>MDRRSFITKAAVGGAAASALAAPALAQSAPKVTWRLASSFPKSLDTIFGGAEVLSKMLSEATDGNFQIQVFSAGELVPGLQAADAVTEGTVECCHTVGYYYWGKDPTFALAAAVPFSLSARGINAWHYHGGGIDLYNEFLSQHNIVAFPGGNTGVQMGGWFRREINTVADMQGLKMRVGGFAGKVMERLGVVPQQIAGGDIYPALEKGTIDATEWVGPYDDEKLGFFKVAPYYYYPGWWEGGPTVHFMFNKSAYEGLTPTYQSLLRTACHAADANMLQLYDWKNPTAIKSLVAQGTQLRPFSPEILQACFEAANEVYAEMEASNPAFKKIWDSIKAFRSEHYTWAQIAEYNYDTFMMVQQNAGKL[4x]

In Rhodobacter sphaeroides, TakP (previously named SmoM) is an ESR from a TRAP transporter and binds α-keto acids in vitro. In this paper, we present the high resolution structures of TakP in its unliganded form and complexed with sodium-pyruvate. This study reveals a key role for an ion in the attachment mode of the substrate, as well as an unexpected dimerization largely mediated by a helix swapping. Thus, and despite very low sequence similarity, the TakP fold is characteristic of a type II ESR.

The structure of the selenomethionine-labeled protein in its native form was first solved by the MAD method and then refined to 2.0 Å resolution with an R-factor of 17.9% (Rfree = 20.5%). For the pyruvate complex all the residues fall in the favored region of the Ramachandran plot whereas in the native one, Trp215 and Val216 are outliers. Our data show that the unliganded TakP was crystallized in the open configuration. This does not exclude the possibility that a more stable closed form might exist in solution, but it makes this hypothesis less likely. Two kinds of conformational changes occur upon complex formation. First, there is a 14° rigid body rotation of domain II (rotation was calculated using the DYNDOM program). Indeed, superimposition of the liganded and unliganded structures results in a r.m.s. deviation of 1.6Å for 334 Cα positions, a value that is an average of a high r.m.s. deviation measured for domain II (3.3Å for 89 Cα positions) and a rather low value for the rest of the molecule, comprising domain I, the clamp and the swapped helix (0.6Å for 245 Cα positions). The dimerization interface is not modified by the open/closed transition, i.e. the intermolecular hydrogen bonds and salt bridges are conserved. The two β-strands hinge allows a rather large rotation of domain II upon ligand binding (from 17° for the Nickel- to 56° for D-ribose- binding proteins; the average is 45°) whereas it is significantly smaller in TakP (14°) and below the average in SiaP (27°). Since the residues responsible for the binding of the substrate belong almost exclusively to domain II, the proximity of the two domains in the apo state may facilitate the substrate-induced closing.ethyl 2-({N-[2-(1H-indol-3-yl)ethyl]glycyl}amino)-4-phenylthiophene-3-carboxylate | C25 H25 N3 O3 S | 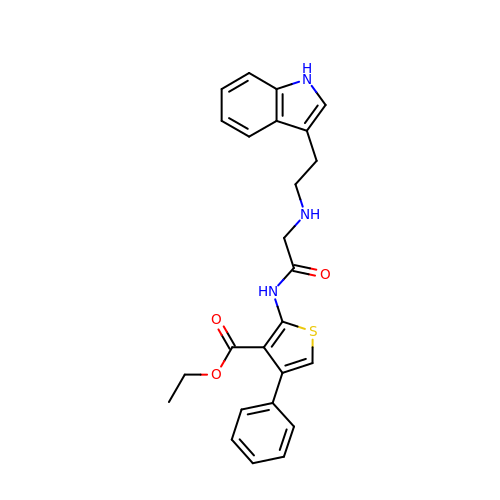VLWAROLSXORELU-UHFFFAOYSA-N>MQRGKVKWFNNEKGYGFIEVEGGSDVFVHFTAIQGEGFKTLEEGQEVSFEIVQG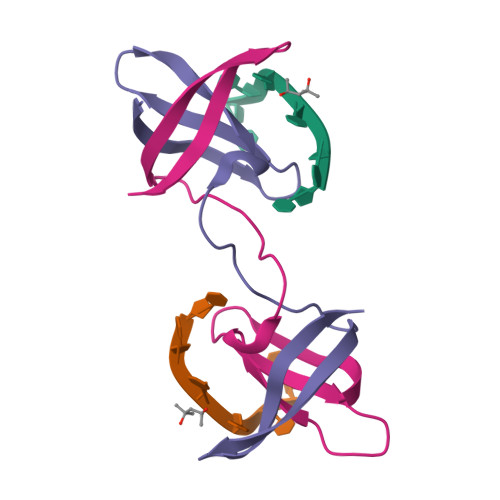NRGPQAANVVKL[2x]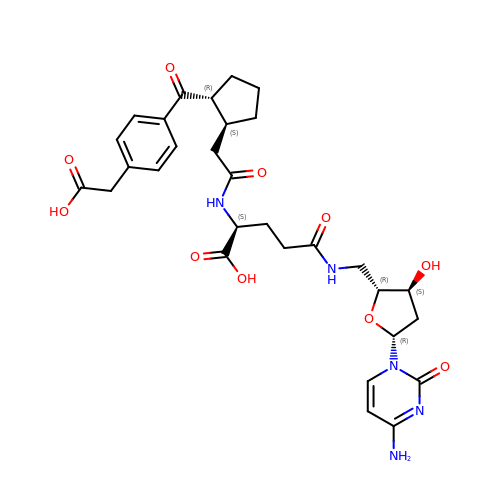5'-{[N-({(1S,2R)-2-[4-(carboxymethyl)benzene-1-carbonyl]cyclopentyl}acetyl)-L-gamma-glutamyl]amino}-2',5'-dideoxycytidine | C30 H37 N5 O10 | JVRVDICAIPFWFZ-BONAQRLYSA-N> MKIYVDGREVIINDNERNLLEALKNVGIEIPNLCYLSEASIYGACRMCLVEINGQITTSCTLKPYEGMKVKTNTPEIYEMRRNILELILATHNRDCTTCDRNGSCKLQKYAEDFGIRKIRFEALKKEHVRDESAPVVRDTSKCILCGDCVRVCEEIQGVGVIEFAKRGFESVVTTAFDTPLIETECVLCGQCVAYCPTGALSIRNDIDKLIEALESDKIVIGMIAPAVRAAIQEEFGIDEDVAMAEKLVSFLKTIGFDKVFDVSFGADLVAYEEAHEFYERLKKGERLPQFTSCCPAWVKHAEHTYPQYLQNLSSVKSPQQALGTVIKKIYARKLGVPEEKIFLVSFMPCTAKKFEAEREEHEGIVDIVLTTRELAQLIKMSRIDINRVEPQPFDRPYGVSSQAGLGFGKAGGVFSCVLSVLNEEIGIEKVDVKSPEDGIRVAEVTLKDGTSFKGAVIYGLGKVKKFLEERKDVEIIEVMACNYGCVGGGGQPYPNDS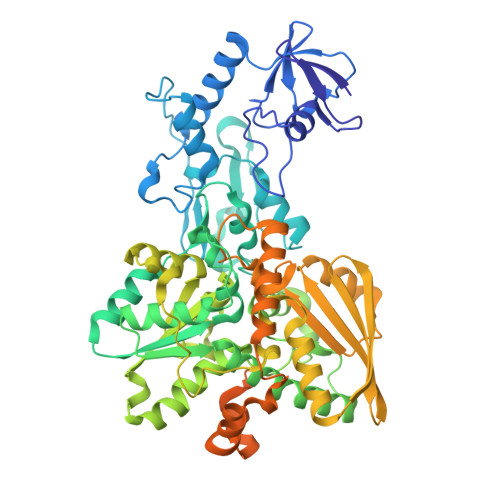RIREHRAKVLRDTMGIKSLLTPVENLFLMKLYEEDLKDEHTRHEILHTTYRPRRRYPEKDVEILPVPNGEKRTVKVCLGTSCYTKGSYEILKKLVDYVKENDMEGKIEVLGTFCVENCGASPNVIVDDKIIGGATFEKVLEELSKNG> GSGVYTVGEFMTKKEDLHVVKPTTTVDEAL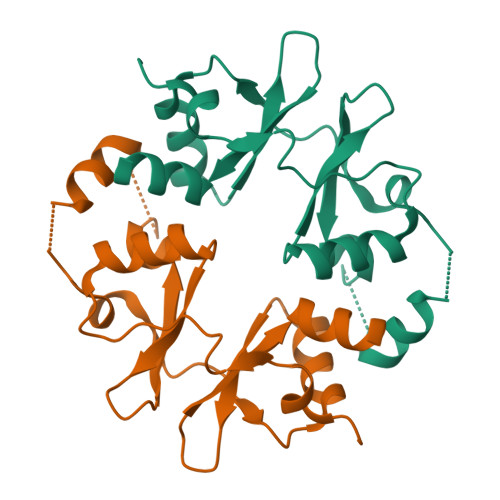ELLVENRITGFPVIDEDWKLVGLVSDYDLLALDSGDSTWKTFNAVQKLLSKTNGKLVGDLMTPAPLVVEEKTNLEDAAKILLETKYRRLPVVDSDGKLVGIITRGNVVRAALQIKRSGDRNA>GPAEAGITGTWSDQLGDTFIVTAGADGALTGTYESAVGNAESRYVLTGRYDSAPATDGSGTALGWTVA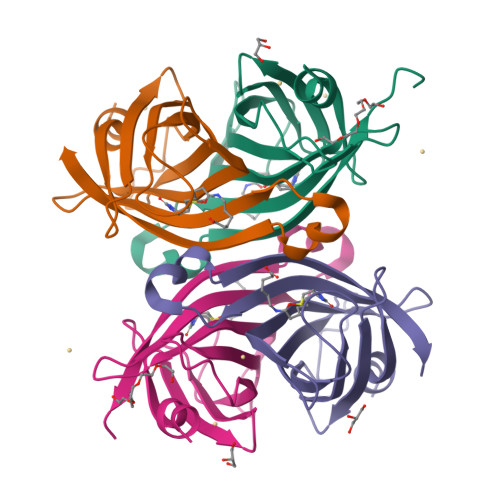WKNNSKNAHSATTWSGQYVGGADAKINTQWLLTSGTTNANAWKSTLVGHDTFTKVKPSAAS[4x]>[2x]MASPSKAVIVPGNGGGDVTTHGWYGWVKKELEKIPGFQCLAKNMPDPITARESIWLPFMETELHCDEKTIIIGHSSGAIAAMRYAETHRVYAIVLVSAYTSDLGDENERASGYFTRPWQWEKIKANCPYIVQFGSTDDPFLPWKEQQEVADRLETKLHKFTDCGHFQNTEFHELITVVKSLLKVPALEHHHHHH

RBBP9 possesses a classical α/β hydrolase superfamily fold, and its hydrolase activity promoted tumour cell proliferation during pancreatic neoplasia. Despite multiple efforts to characterize the cellular activity of RBBP9, its enzymatic function in cells has remained enigmatic. Finally, we develop a pipeline to directly identify the branched peptides formed between a substrate fragment and Dap and thereby reveal that the putative serine hydrolase retinoblastoma binding protein 9 (RBBP9) is an aminopeptidase with a preference for removing aromatic amino acids in mammalian cells. Overall, our results demonstrate that RBBP9 is an aminopeptidase with a preference for removing aromatic residues from the N terminus in human cells.

Collectively, we demonstrated that RBBP9(S75Dap) preferentially forms conjugates with individual hydrophobic amino acids. RBBP9 showed a clear preference for hydrolysing aromatic residues, especially Phe and Tyr; this is generally consistent with the mass adducts identified on Dap from live cells. Moreover, RBBP9-mediated hydrolysis required a free α-amine, as acetylated Met–AMC (AcMet–AMC) and the dipeptide Glu-Phe–AMC were not hydrolysed; this explains why the aminopeptidase activity was not detected even though a subset of protease substrates (for example, Pro–pNA and Suc-Phe–pNA) were screened in previous studies. To understand the preference shown by RBBP9 towards aromatic residues, we solved the crystal structure of RBBP9 in complex with Phe. The overall structure of this complex is almost identical (root mean squared deviation = 0.17 Å) to that of RBBP9 alone. Phe sits in the RBBP9 catalytic pocket. Tyr99, Leu103, Phe140 and Leu141 form a hydrophobic cage that holds the bulky aromatic ring of Phe in position. In addition, the hydrogen bond formed between the α-amine of Phe and the side chain of Glu108 (or Ser76 or Tyr99) anchors the amino group at this position; this explains why a free α-amine is required on the N terminus of RBBP9 substrates.> GHMSHLADVSPPTACRVCGGGVQEFLDLGRQPLSDRFRKPDELDDEFTYRLAVGRCDSCEMVQLTEEVPRDLMFHEVYPYHSSGSSVMREHFAMLARDFLATELTGPDPFIVEIGCNDGIMLRTIQEAGVRHLGFEPSSGVAAKAREKGIRVRTDFFEKATADDVRRTEGPANVIYAANTLCHIPYVQSVLEGVDALLAPDGVFV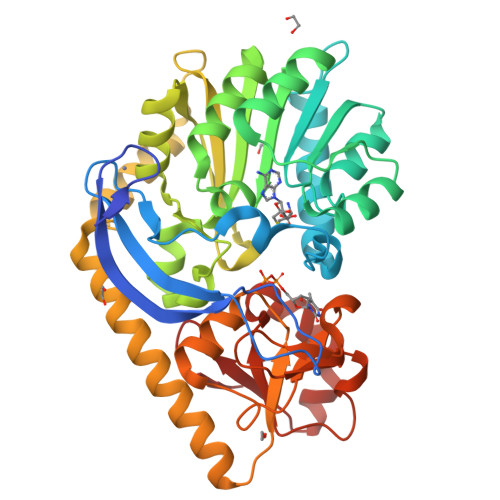FEDPYLGDIVAKTSFDQIFDEHFFLFSATSVQGMAQRCGFELVDVQRLPVHGGEVRYTLARQGSRTPSAAVAQLLAAEREQELSDMATLRAFAGNVVKIRDELTALLHRLRAEGRSVVGYGATAKSATVTNFCGIGPDLVHSVYDTTPDKQNRLTPGAHIPVRPASAFSDPYPDYALLFAWNHAEEIMAKEQEFHQAGGRWILYVPEVHIR2,2'-{benzene-1,3-diylbis[ethyne-2,1-diyl(5-bromobenzene-3,1-diyl)]}diethanamine | C26 H22 Br2 N2 | 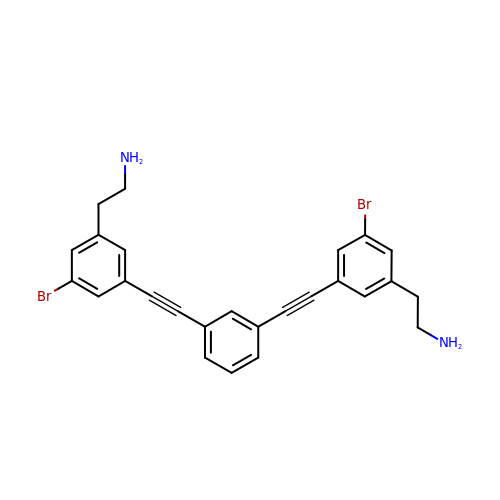JSVQCKAPBSOZCB-UHFFFAOYSA-N> NLRQAVMLPEGEDLNEWIAVN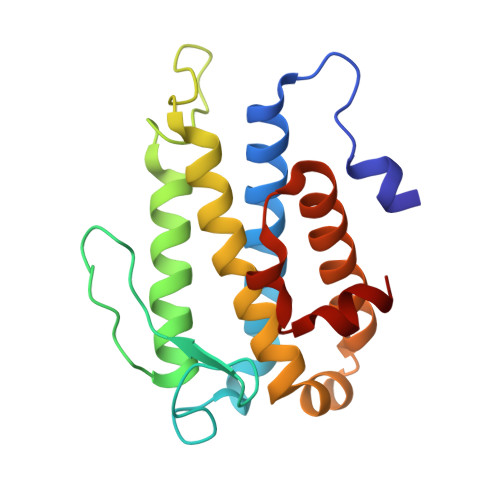TVDFFNQINMLYGTITEFCTEASCPVMSAGPRYEYHWADGTNIKKPIKCSAPKYIDYLMTWVQDQLDDETLFPSKIGVPFPKNFMSVAKTILKRLFRVYAHIYHQHFDSVMQLQEEAHLNTSFKHFIFFVQEFNLIDRRELAPLQELIEKL>[30x]AAGQGKA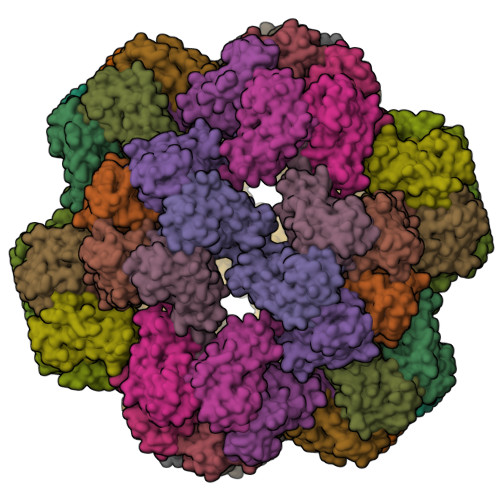IKAIAGYSISKWEASSDAITAKATNAMSITLPHELSSEKNKELKVGRVLLWLGLLPSVAGRIKACVAEKQAQAEAAFQVALAVADSSKEVVAAMYTDAFRGATLGDLLNLQIYLYASEAVPAKAVVVHLEVEHVRPTFDDFFTPVYR> MGSMEAERVRVFHKQAFEYISIALRIDEDEKAGQKEQA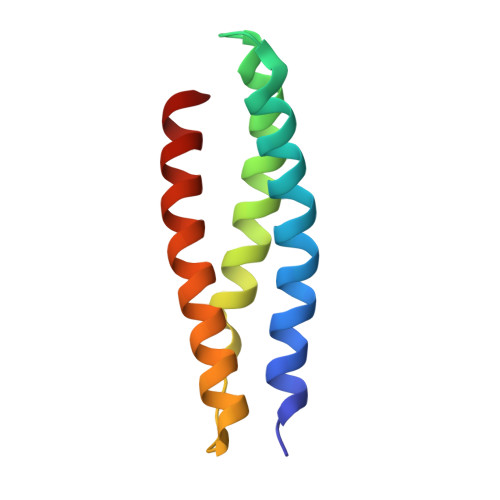VEWYKKGIEELEKGIAVIVTGQGEQCERARRLQAKMMTNLVMAKDRLQLLE> KSPIFGPQEVSSIEGDSVSITCYYPDTSVNRHTRKYWCRQGASGMCTTLISSNGYLSK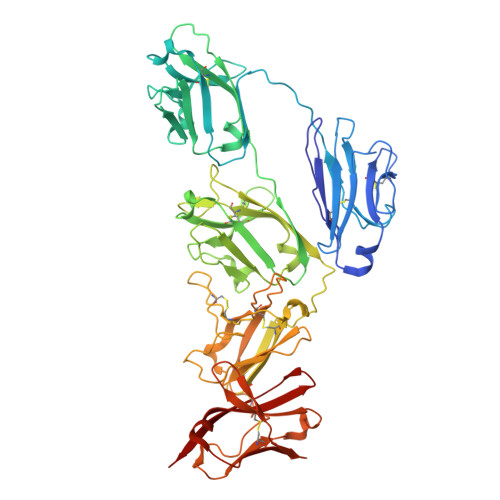EYSGRANLINFPENNTFVINIEQLTQDDTGSYKCGLGTSNRGLSFDVSLEVSQVPELPSDTHVYTKDIGRNVTIECPFKRENAPSKKSLCKKTNQSCELVIDSTEKVNPSYIGRAKLFMKGTDLTVFYVNISHLTHNDAGLYICQAGEGPSADKKNVDLQVLAPEPELLYKDLRSSVTFECDLGREVANEAKYLCRMNKETCDVIINTLGKRDPDFEGRILITPKDDNGRFSVLITGLRKEDAGHYQCGAHSSGLPQEGWPIQTWQLFVNEESTIPNRRSVVKGVTGGSVAIACPYNPKESSSLKYWCRWEGDGNGHCPVLVGTQAQVQEEYEGRLALFDQPGNGTYTVILNQLTTEDAGFYWCLTNGDSRWRTTIELQVAEATREPNLEVTPQNATAVLGETFTVSCHYPCKFYSQEKYWCKWSNKGCHILPSHDEGARQSSVSCDQSSQLVSMTLNPVSKEDEGWYWCGVKQGQTYGETTAIYIAVEER>[4x]SDDLSFKFKNFSQNGKDLSFQGNASVIETGVLQLNKVGNNLPDETGGIARYIAPIHIWNCNTGELASFITSFSFFMETSANPKAATDGLTFFLAPPD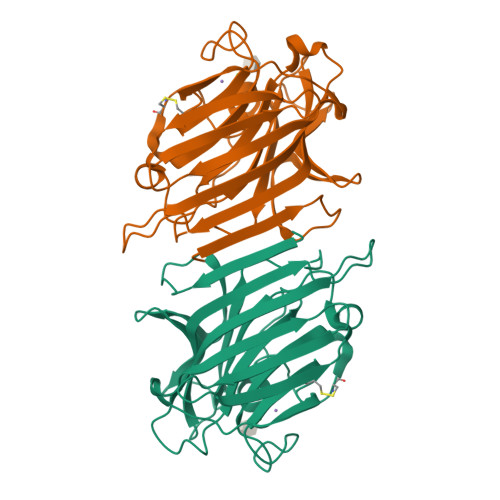SPLRRAGGYFGLFNDTKCDSSYQTVAVEFDTIGSPVNFWDPGFPHIGIDVNCVKSINAERWNKRYGLNNVANVEIIYEASSKTLTASLTYPSDQTSISVTSIVDLKEILPEWVSVGFSGSTYIGRQATHEVLNWYFTSTFINTNS>[2x]MFKNLIWLKEVDSTQERLKEWNVSYGTALVADRQTKG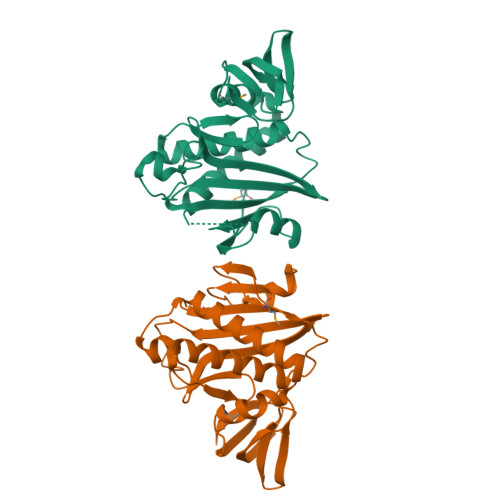RGRLGRKWLSQEGGLYFSFLLNPKEFENLLQLPLVLGLSVSEALEEITEIPFSLKWPNDVYFQEKKVSGVLCELSKDKLIVGIGINVNQREIPEEIKDRATTLYEITGKDWDRKEVLLKVLKRISENLKKFKEKSFKEFKGKIESKMLYLGEEVKLLGEGKITGKLVGLSEKGGALILTEEGIKEILSGEFSLRRS> GNPTPKSCTVSEEDLTTIRNAIQKASRASLDDVNLDEDLIAKCPLLKTITASLKSVASEIATLKDTGISEEQVDELKQSYEQQVNEIVKSRDIFEKQSGGDVMKEQGAMINRMTELQVQVAQLQQQIGEQTSRMYDDMAELIFQRLAMNSTDSIRNYTAHMMEQKLHTLMTKLETNYRIFLGALRYLDHLGDQPLIDKVFDGILKRLDEMSLETNKERENGKYVLVNLLCWTVNNRFLTEKYRKK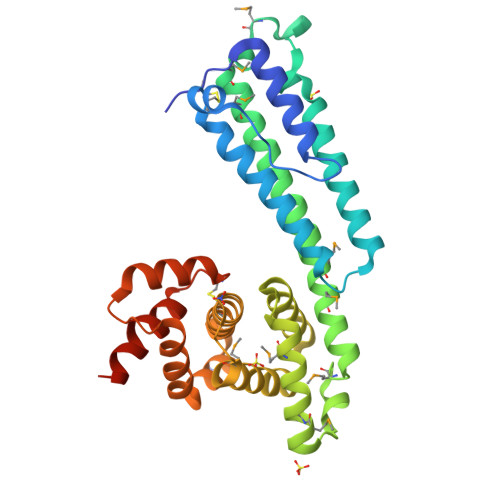QLELFRIALKFYPKTGNKEANEADIRGRQFCDANFPVNVITWFAVSRAAEGWGLRGTLAAA> NRRNKARKVVSRSTALVPMAPASQRTGPAPRKPRKRNQALVRNPRLTDAGLAFLKCAFAAPDFSVDPGKGIPDNFHGRTLAIKDCNTTSVVFTPNTDTYIVVAPVPGFAYFRAEVAVGAQPTTFVGVPYPTYATNFGAGSQNGLPAVNNYSKFRYASMACGLYPTSNMMQFSGSVQVWRVDLNLSEAVNPAVTAITPAPGVFANFVDKRINGLRGIRPLAPRDNYSGNFIDGAYTFAFDKSTDFEWCD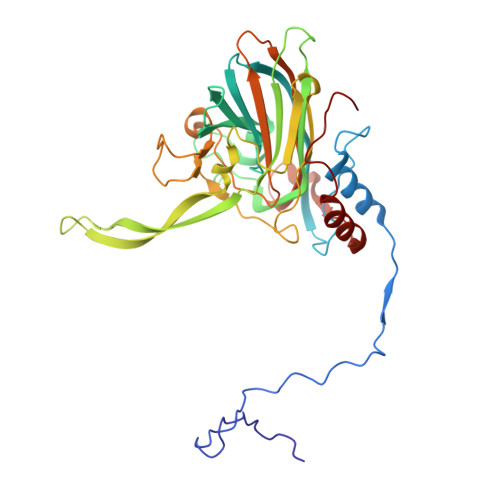FVRSLEFSESNVLGAATAMKLLAPGGGTDTTLTGLGNVNTLVYKISTPTGAVNTAILRTWNCIELQPYTDSALFQFSGVSPPFDPLALECYHNLKMRFPVAVSSREN>LKENPSGRPRSKEGDKGCGALVWVGEPVTLRTAETIAGKYGVWMRDPKPTHPYTQESTWRIDTVGTEIRQVFEYSQISQFEQGYPSKVHVLPRALESTGAVVYAGSLYFQGAESRTVVRYELDTETVKAEKEIPGAGYHGHFPYAWGGYTDIDLAVDESGLWVIYSTEEAKGAIVLSKLNPANLELERTWETNIRKQSVANAFVICGILYTVSSYSSAHATVNFAYDTKTGTSKTLTIPFTNRYKYSSMIDYNPLERKLFAWDNFNMV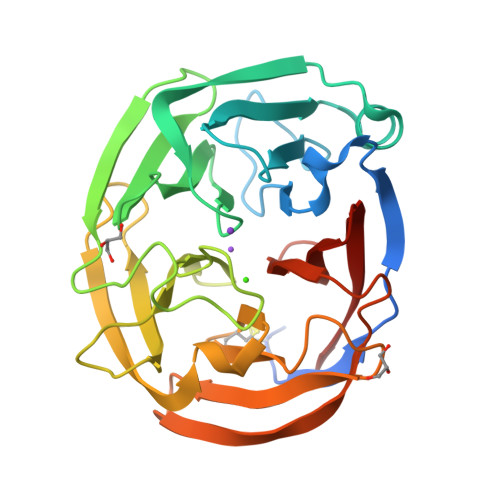TYDIKLLEM[2x]> MMQQSRPASDPQVVEAARKEGRLIIYSSTDQSSAQALLDDFRKLYPFIQIEYNDLGTQAIYDRFVSETAAGASSADLLWSSAMELQVKLASEGYALPYDSPEAKNWPANARLGNLAYSTTLEPAVVVYNKRFLKPEEVPTTREGLARLLQEPRMRGRVATWDPERAAVGFTILKADYDRFPAFQELARAFGKAQAALYSSTGAAFEKVISGEHYLAYGFFGSYALLRQRTVKDLGIAYLT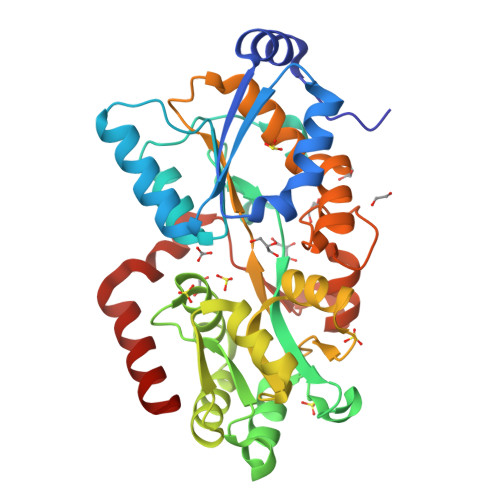DGTVAIQRVAFINKRAAHPNAAKLFLDYLLSLRGQNLMAYTALIFARRETVVGEATPQALYKAVGGKDKVYAIPVSTEILKNLDPAERMRFLTFWRQAVRGQ> GAMGSMVKLAEFSRTATFAWSHDKIPLLVSGTVSGTVDANFSTDSSLELWSLLAADSEKPIASLQVDSKFNDLDWSHNNKIIAGALDNGSLELYSTNEANNAINSMARFSNHSSSVKTVKFNAKQDNVLASGGNNGEIFIWDMNKCTESPSNYTPLTPGQSMSSVDEVISLAWNQSLAHVFASAGSSNFASIWDLKAKKEVIHLSYTSPNSGIKQQLSVVEWHPKNSTRVATATGSDNDPSILIWDLRNANTPLQTLNQGHQKGILSLDWCHQDEHLLLSSGRDNTVLLWNPESAEQLSQFPARGNWCFKTKFAPEAPDLFACASFDNKIEVQTLQNLTNTLDEQETETKQQESETDFWNNVSREESKEKPSVFHLQAPTWYGEPSPAAHWAFGGKLVQITPDGKGVSITNPKISG;> MVVIANA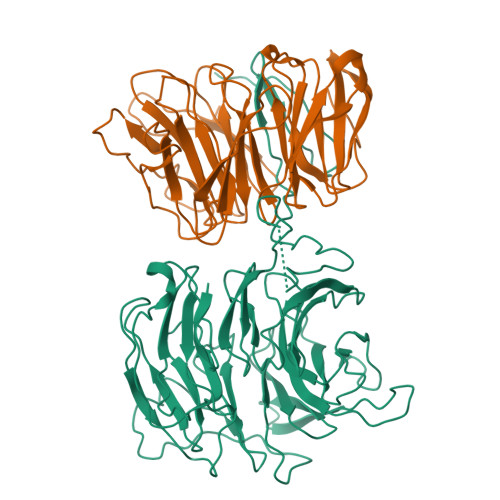HNEMIHDAVMDYYGKRMATCSSDKTIKIFEVEGETHKLIDTLTGHEGPVWRVDWAHPKFGTILASCSYDGKVMIWKEENGRWSQIAVHAVHSASVNSVQWAPHEYGPMLLVASSDGKVSVVEFKENGTTSPIIIDAHAIGVNSASWAPATIEEDGEHNGTKESRKFVTGGADNLVKIWKYNSDAQTYVLESTLEGHSDWVRDVAWSPTVLLRSYMASVSQDRTCIIWTQDNEQGPWKKTLLKEEKFPDVLWRASWSLSGNVLALSGGDNKVTLWKENLEGKWEPAGEVHQ> HHEADRIPVVLDNPPWAKPFELLVSFLNTPKYGTFDPTPVVPVFFPFWFGMIVGDIGYALLFYLVGRWLSGYVKRNEPLVIDLFALKLKPQVIGKLVHILNWMVFWTVVWGVIYGEFFGTFLEHLGVFGTPEHPGLIPILIHRIDTAKTANLLILLSVAFGVVLVFFGLALRAYLGLKHRHMAHFWEGVGYLGGLVGVLALAASYLGNLQAGWLQGLMYLGFGVFLLAVLMSRIWLMIPEI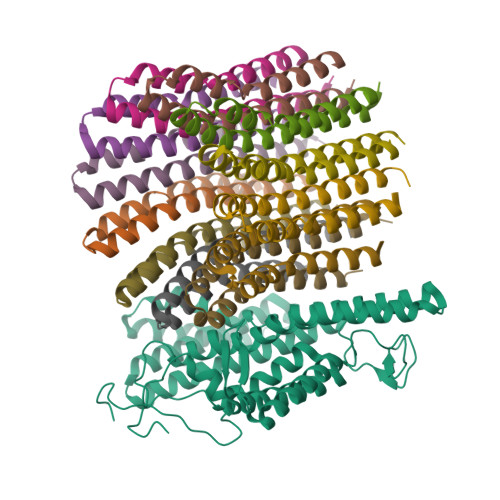FTQAGHILSHIRIYAVGAAGGILAGLLTDVGFALAERLGLLGVLLGLLVAGVLHLLILLLTTLGHMLQPIRLLWVEFFTKFGFYEENGRPYRPFKSVR;>[12x]SGGLDRGLIAVGMGLAVGLAALGTGVAQARIGAAGVGAIAEDRSNFGTALIFLLLPETLVIFGLLIAFILNGRL> MGKYNLILSEYLSFIYNSQSAVQIPIYYSSNSELENRCIEFHSKCLENSKNGLSLKKLFVEYSDVIENATLLSILSYSYDKYNAVERKLVKYAKGKPLEADLTVNELDYENNKITSELFPTAEEYTDLLMDPAILTSLSSNLNAVMFWLEKHENDVAEKLKIYKRRLDLFTIVASTVNKYGVPRHNAKYRYEYEVMKDKPYYLVTWANSSIEMLMSVFSHEDYLIARELIVLSYSNRSTLAKLVSSPMSILVALVDINGTFITNEELELEFSNKYVRAIVPDQTFDELKQMLDNMRKAGLTDIPKMIQDWLVDCSIEKFPLMAKIYSWSFHVGFRKQKMLDAALDQLKTEYTEDVDDEMYREYTMLIRDEVVKMLEEPVKHDDHLLQDSELAGLLSMSSASNGESRQLKFGRKTIFSTKKNMHVMDDMANGRYTPGIIPPVNVDKPIPLGRRDVPGRRTRIIFILPYEYFIAQHAVVEKMLIYAKHTREYAEFYSQSNQLLSYGDVTRFLSNNSMVLYTDVSQWDSSQHNTQPFRKGIIMGLDMLANMTNDARVIQTLNLYKQTQINLMDSYVQIPDGNVIKKIQYGAVASGEKQTKAANSIANLALIKTVLSRISNKYSFATKIIRVDGDDNYAVLQFNTEVTKQMVQDVSNDVRETYARMNTKVKALVSTVGIEIAKRYIAGGKIFFRAGINLLNNEKKGQSTQWDQAAVLYSNYIVNRLRGFETDREFILTKIMQMTSVAITGSLRLFPSERVLTTNSTFKVFDSEDFIIEYGTTDDEVYIQRAFMSLSSQKSGIADEIAASSTFKNYVSRLSEQLLFSKNNIVSRGIALTEKAKLNSYAPISLEKRRAQISALLTMLQKPVTFKSSKITINDILRDIKPFFTVNEAHLPIQYQKFMPTLPDNVQYIIQCI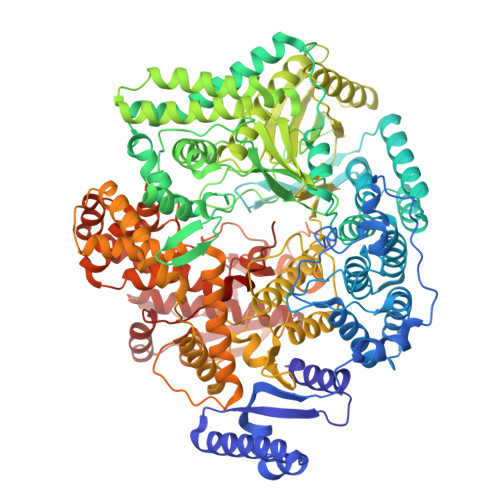GSRTYQIEDDGSKSAISRLISKYSVYKPSIEELYKVISLHENEIQLYLISLGIPKIDADTYVGSKIYSQDKYRILESYVYNLLSINYGCYQLFDFNSPDLEKLIRIPFKGKIPAVTFILHLYAKLEVINHAIKNGSWISLFCNYPKSEMIKLWKKMWNITSLRSPYTNANFFQD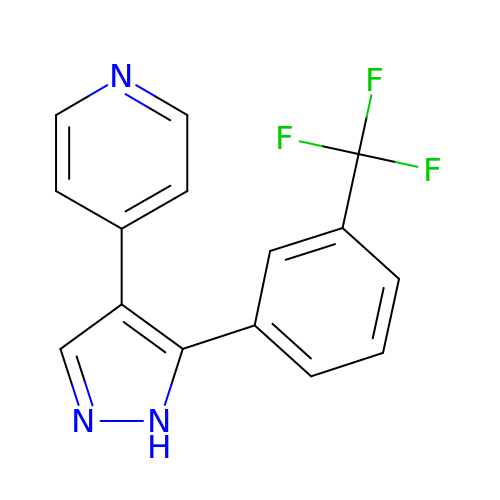4-[5-[3-(trifluoromethyl)phenyl]-1H-pyrazol-4-yl]pyridine | C15 H10 F3 N3 | UZOPNNYVHHABCA-UHFFFAOYSA-N>MNHKVHHHH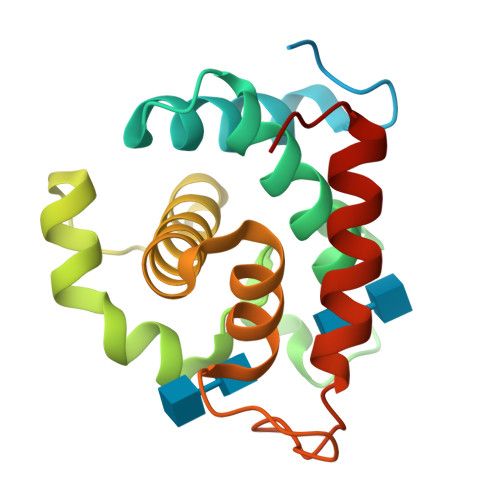HHIEGRHMGTTPSDPPTNPPTTVTKPAEVPSRIWTYVMNADNAYGKGGDFALLLSAVIKKESYFGDGLSGSPSAGDGLMQVQPNTRNAYLSQFSAKYGHAYNHSSEQDQVYMGSLILNEKIVRFGSIYSGLLHYNGGDYWYPGATDSYGRPILADQYANTVYAQYKSYGGRYSR[4x]>GMSSNLHGIAIGIERSQDDFYLAFKAVGKLTHEDYEQMTPLLESALAGIKTPEIVALIDITELDGLSLHAAWDDLKLGLKHGKEFKRVAIIGQGELQEWATRVANWFTPGEFKFFEDKRDALDWLC[2x]

The crystal structures of the proteins encoded by the YP_749275.1 and YP_001095227.1 genes from Shewanella frigidimarina and S. loihica, respectively, have been determined at 1.8 and 2.25 Å resolution, respectively. These proteins are members of a novel family of bacterial proteins that adopt the α/β SpoIIAA-like fold found in STAS and CRAL-TRIO domains.

An ortholog with 54% sequence identity from S. loihica (YP_001095227.1) is also of unknown function, with a molecular weight of 14 105 Da (residues 1–125) and a calculated isoelectric point of 4.9. Similarly, the structure of YP_001095227.1 consists of a protein dimer (residues 0–125 for chain A and residues 0–48 and 53–125 for chain B), two sodium ions, two chloride ions, nine 2-methyl-2,4-pentanediol molecules and 95 water molecules in the asymmetric unit. In the ‘open’ conformation (YP_001095227.1), these helices are 15 Å apart, leading to the creation of a deep nonpolar cavity. An analysis using the CastP server reveals a deep cavity (1743 Å3) lined by over 20 residues that are all hydrophobic, except for Asp73, which is hydrogen bonded to Tyr34. The floor of the cavity is formed by the β-sheet and helix α1. This large hydrophobic cavity represents a potential ligand-binding pocket that is occupied in the crystal structure by three 2-methyl-2,4-pentanediol (MPD) molecules, which are likely to stabilize the ‘open’ conformation by partially filling the cavity. Conversely, in the ‘open’ state, Trp71 is solvent-exposed and may participate in protein–membrane interactions, whereas His6 and His31 form stabilizing hydrogen bonds with Asp33 and Asp72, respectively. The dimerization mode of the ‘open’ structure, YP_001095227.1, is different and comparatively weaker. The presence of a deep cavity in YP_001095227.1 is similar to the eukaryotic Sec14-like proteins, which also adopt the same SpoIIAA-like fold. Calculations using the PPM method show that the ‘open’ conformation of YP_001095227.1 can associate with the lipid bilayer by immersing its exposed nonpolar residues from α2 and α3 into the lipid acyl-chain region.> PEGD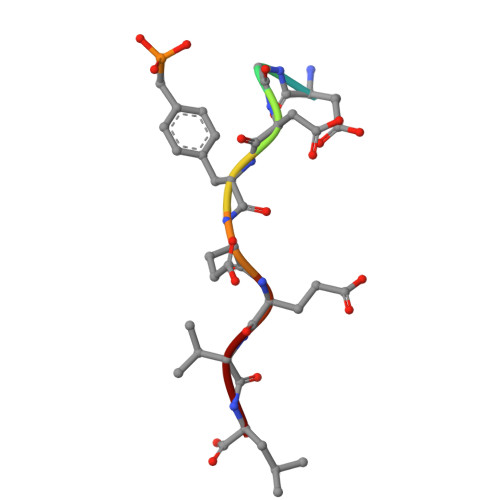FEEVL> MALTNNLWAFVFGILGNIISFVLFLAPVPTFVRICKKKSTEGFQSLPYVSALFNAMLWIYYAMQKDGTAFLLITINAFGCVIETIYIVLFVSYANKKTRISTLKVLGLLNFLGFAAIVLVCELLTKGSTREKVLGGICVGFSVSMFAAPLSIMRVVVRTRSVEFMPFSLSL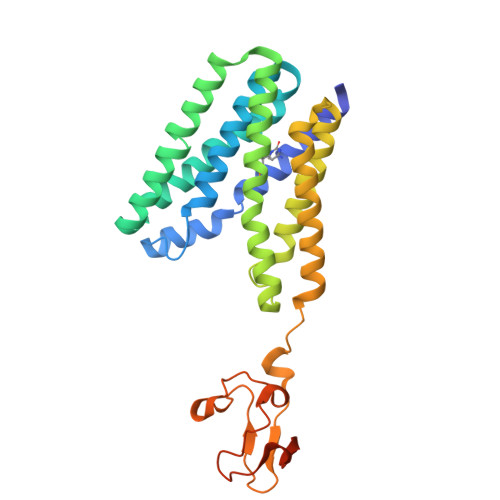FLTINAVTWLFYGLAIKDFYVALPNVLGAFLGAVQMILYIIFKYYKTPVAQMKKYTCTVCGYIYNPEDGDPDNGVNPGTDFKDIPDDWVCPLCGVGKDQFEEVEEENLYFQGHHHHHHHHHH>TADELVFFVNGKKVVEKNADPETTLLAYLRRKLGLRGTKLGCGEGGCGACTVMLSKYDRLQDKIIHFSANACLAPICTLHHVAVTTVEGIGSTKTRLHPVQERIAKSHGSQCGFCTPGIVMSMYTLLRNQPEPTVEEIEDAFQGNLCRCTGYRPILQGFRTFAK[2x];>[2x]LFNPEEFMPLDPTQEPIFPPELLRLKDVPPKQLRFEGERVTWIQASTLKELLDLKAQHPEAKLVVGNTEIGIEMKFKNQLFPMIICPAWIPELNAVEHGPEGISFGAACALSSVEKTLLEAVAKLPTQKTEVFRGVLEQLRWFAGKQVKSVASLGGNIITASPISDLNPVFMASGTKLTIVSRGTRRTVPMDHTFFPSYRKTLLGPEEILLSIEIPYSREDEFFSAFKQASRREDDIAKVTCGMRVLFQPGSMQVKELALCYGGMADRTISALKTTQKQLSKFWNEKLLQDVCAGLAEELSLSPDAPGGMIEFRRTLTLSFFFKFYLTVLKKLG;>DTVGRPLPHLAAAMQASGEAVYCDDIPRYENELFLRLVTSTRAHAKIKSIDVSEAQKVPGFVCFLSADDIPGSNETGLFNDETVFAKDTVTCVGHIIGAVVADTPEHAERAAHVVKVTYEDLPAIITIEDAIKNNSFYGSELKIEKGDLKKGFSEADNVVSGELYIGGQDHFYLETHCTIAIPKGEEGEMELFVSTQNAMKTQSFVAKMLGVPVNRILVRVKRMGGGFGGKETRSTLVSVAVALAAYKTGHPVRCMLDRNEDMLITGGRHPFLARYKVGFMKTGTIVALEVDHYSNAGNSRDLSHSIMERALFHM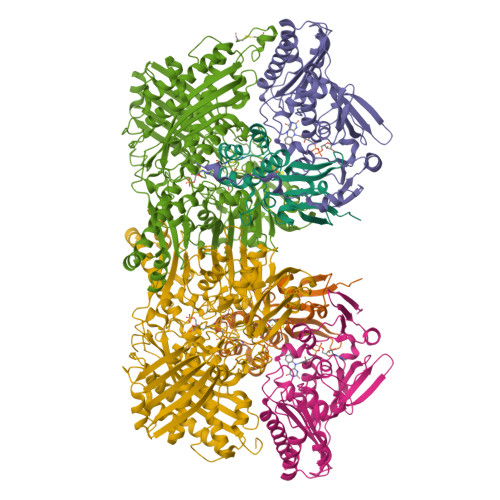DNCYKIPNIRGTGRLCKTNLSSNTAFRGFGGPQALFIAENWMSEVAVTCGLPAEEVRWKNMYKEGDLTHFNQRLEGFSVPRCWDECLKSSQYYARKSEVDKFNKENCWKKRGLCIIPTKFGISFTVPFLNQAGALIHVYTDGSVLVSHGGTEMGQGLHTKMVQVASKALKIPISKIYISETSTNTVPNSSPTAASVSTDIYGQAVYEACQTILKRLEPFKKKNPDGSWEDWVMAAYQDRVSLSTTGFYRTPNLGYSFETNSGNAFHYFTYGVACSEVEIDCLTGDHKNLRTDIVMDVGSSLNPAIDIGQVEGAFVQGLGLFTLEELHYSPEGSLHTRGPSTYKIPAFGSIPTEFRVSLLRDCPNKKAIYASKAVGEPPLFLGASVFFAIKDAIRAARAQHTNNNTKELFRLDSPATPEKIRNACVDKFTTLCVTGAPGNC[2x]>GSHMSEWKARRFWASVGIHKEEGGWAVLLDERPLRTPGKQPLRLPTEALALAIAEEWQAVQEVIDPNAMPLTRSANSAIEKVAPQFDAVAAMLGDYGGTDLLSYRADAPEALVRAQAEGWDPLIDWAATELRAPLRITHGVIPVPQDPVVLLKL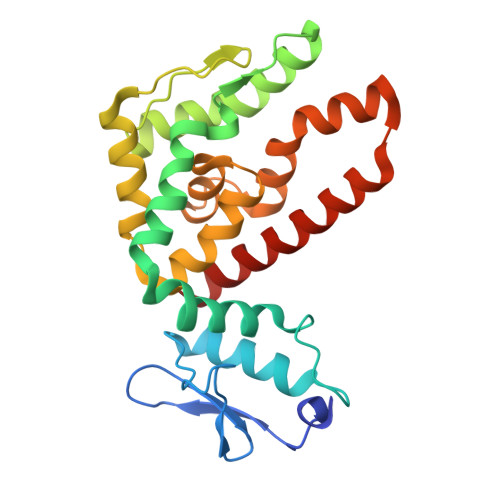RAEVASLDPFGLTALHDLVTLPGSLILGLAVIRGRIDAPTAHALSRIDEEFQAERWGRDEEAEAQAASRLAAMRDSERFWHLTRG[2x]> GSGSAKYTYRSLGRHLDFLRPGLRFGGSQSSKYTYYTVEVKIDTVNLPLYKDSRSLDPHVTGTFTIKNLTPVLDKVVTLFEGYVINYNQFPLCSLHWPAEETLDPYMAQRESDCSHWKRFGHFGSDNWSLTERNFGQYNH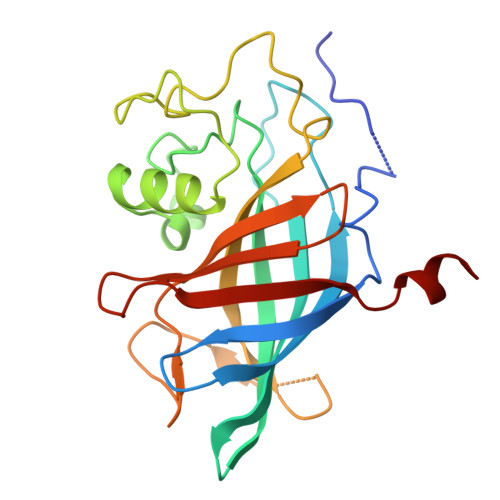ESAEFMNQRYIYLKWKERFLLDDEEQENLMLDDNHHLEGASFEGFYYVCLDQLTGSVEGYYYHPACELFQKLELVPTNCDALNT> MGTQQKDVTIKSDAPDTLLLEKHADYIASYGSKKDDYEYCMSEYLRMSGVYWGLTVMDLMGQLHRMNKEEIL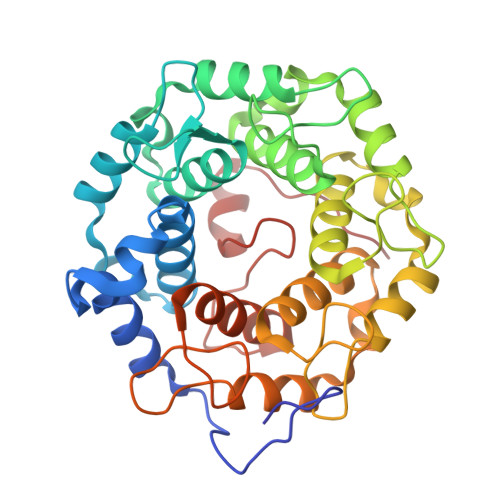VFIKSCQHECGGVSASIGHDPHLLYTLSAVQILTLYDSIHVINVDKVVAYVQSLQKEDGSFAGDIWGEIDTRFSFCAVATLALLGKLDAINVEKAIEFVLSCMNFDGGFGCRPGSESHAGQIYCCTGFLAITSQLHQVNSDLLGWWLCERQLPSGGLNGRPEKLPDVCYSWWVLASLKIIGRLHWIDREKLRSFILACQDEETGGFADRPGDMVDPFHTLFGIAGLSLLGEEQIKPVSPVFCMPEEVLQRVNVQPELVS> MSKTTPTKDSIRAEFEELVEKDSFWSKFVGSQFVSMLTLFITQIVYRCFQYADAALAEGFISTATRRSSILAAAETNSYVGTKPTPSSGMIEITATSEDAPAVIPKNMPLISDDQYPYMTMDVCRLVDGTGTVEVAQLEIQEVTYTVTAAKEFLEVVLSKALTAVCYKLEVFVTTDGKTTQWSSSTMFRLAGSKSQVYVEFYKPSEQLGVRFGDGLIGQIPPEGSTITLKVWCTNGDITLVAGQNLTPVDSAANLANLISVKTTTPITAGTDAETTEITRNRAQYYLAYDDQVVWGGDYTYFLVRNIPGLSWVKAWGEGQQEKLDGAYNVQNINKIFISGWHPNKSQSELEEMILAAFKKVPNELNKKFSYKEVRKLPFKITITGRISASLTIENVTDELKSALETKFGRDSTFFDPNRVGKYILIKKKDVWAFIETLGYFRDFYLEFVEWN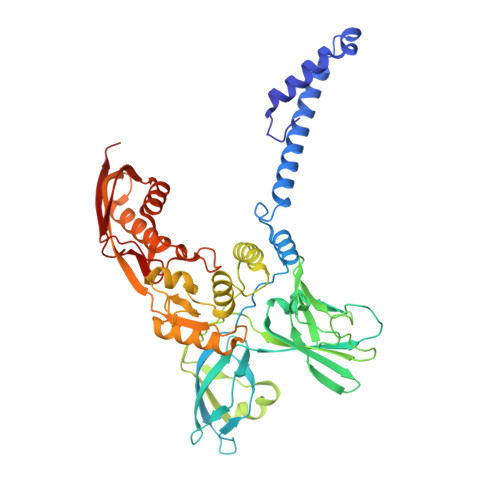ESNGFYDFVYLDTENSTFNISYEEE>[2x]MTKHYDYIAIGGGSGGIASINRAAMYGQKCALIEAKELGGTCVNVGCVPKKVMWHAAQIREAIHMYGPDYGFDTTINKFNWETLIASRTAYIDRIHTSYENVLGKNNVDVIKGFARFVDAKTLEVNGETITADHILIATGGRPSHPDIPGVEYGIDSDGFFALP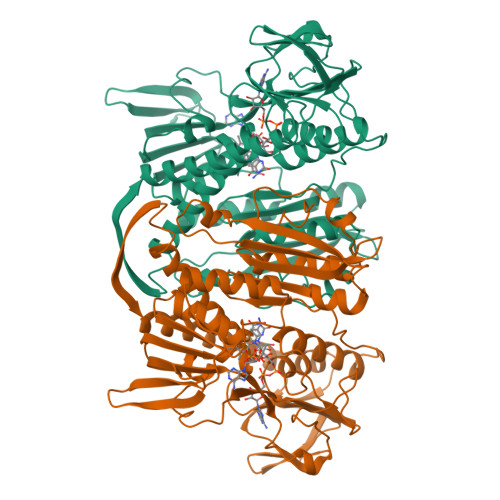ALPERVAVVGAGYIAVELAGVINGLGAKTHLFVRKHAPLRSFDPMISETLVEVMNAEGPQLHTNAIPKAVVKNTDGSLTLELEDGRSETVDCLIWAIGREPANDNINLEAAGVKTNEKGYIVVDKYQNTNIEGIYAVGDNTGAVELTPVAVAAGRRLSERLFNNKPDEHLDYSNIPTVVFSHPPIGTVGLTEPQAREQYGDDQVKVYKSSFTAMYTAVTTHRQPCRMKLVCVGSEEKIVGIHGIGFGMDEMLQGFAVALKMGATKKDFDNTVAIHPTAAEEFVTMR The Nucleoside diphosphate linked to another moiety, X (Nudix) superfamily of proteins constitute pyrophosphohydrolases of substrates that include (d)NTPs, nucleotide sugars, capped (m7Gppp and Gppp) RNAs and dinucleotide coenzymes including NAD, FAD, dephosphoCoA (dpCoA) and their derivatives. Among the Nudix proteins, Nudt16 is the most promiscuous. Similar to DXO, it can hydrolyze RNAs harboring an m7G cap, unmethylated cap, NAD cap, dpCoA cap and FAD cap on the 5′end. To understand the molecular mechanism for the recognition of FAD-capped RNA by Nudt16, we determined the crystal structure of human Nudt16 in complex with FAD at 2.7 Å resolution and the structure of free human Nudt16 at 2.3 Å resolution.

The overall structure of Nudt16 is similar to those reported earlier, with rms distances of approximately 0.6 Å for the dimer. The loop containing residues 101–106, located near the ribose of FAD in the complex, shows substantial variations among the structures and has weak electron density in the free Nudt16 structure.

>MAGARRLELGEALALGSGWRHACHALLYAPDPGMLFGRIPLRYAILMQMRFDGRLGFPGGFVDTQDRSLEDGLNRELREELGEAAAAFRVERTDYRSSHVGSGPRVVAHFYAKRLTLEELLAVEAGATRAKDHGLEVLGLVRVPLYTLRDGVGGLPTFLENSFIGSAREQLLEALQDLGLLQSGSISGLKIPAHH[4x]> GSHMDSLRPKLSEEQQRIIAILLDAHHKTYDPTYSDFCQFRPPVRVNDGGGSVTLELSQLSMLPHLADLVSYSIQKVIGFAKMIPGFRDLTSEDQIVLLKSSAIEVIMLRSNESFTMDDMSWTCGNQDY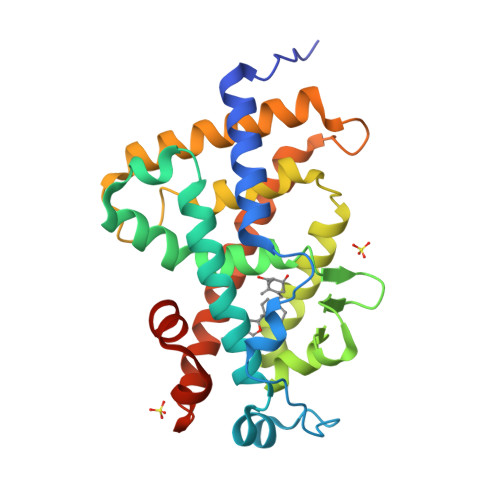KYRVSDVTKAGHSLELIEPLIKFQVGLKKLNLHEEEHVLLMAICIVSPDRPGVQDAALIEAIQDRLSNTLQTYIRCRHPPPGSHLLYAKMIQKLADLRSLNEEHSKQYRCLSFQPECSMKLTPLVLEVFGNEIS> MSVQIGNGLLMVVAPGTLTVGSARARLIRQVTLADFCEPQAERPGLVVLALRHPADLAGAAYAATPPGKNHRDLEEAWLALDEGGRGLGGDGIRASVVSLNFLVAAAENADDALRAHVTTNYRDRRTAARLERFATVLRAMIRSHVFPHRALHVLGGLLGHVTQDRLASVTCVARGDQEAARTNDMAARRSQVHVPACALMDVDRELRLGGDDGLRFAYLVFVYTQRHRREALRVHVAVSRLPELGDALSFLLAGTRVDNAIHGTDEAD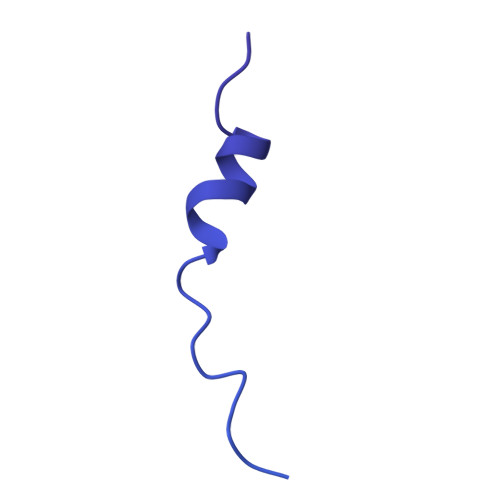APAAPAAAAAFPAYLFNDPRSARCPTGRLNTPAAEALPVWAPDMRGRATRNSCMYAAYVRLGTVERVVRRAERCGSVDLPLAHMERFTWDVGAWEECFF>[2x]MFKFIGCGSAFNTRLGNNSAYIKEDGILFMIDCGSANFDRIMRSDLLEGVEDIVVLMTHTHPDHVGSLGDLIFYSYFCMGQVKVPNLTVYAPYDMKIS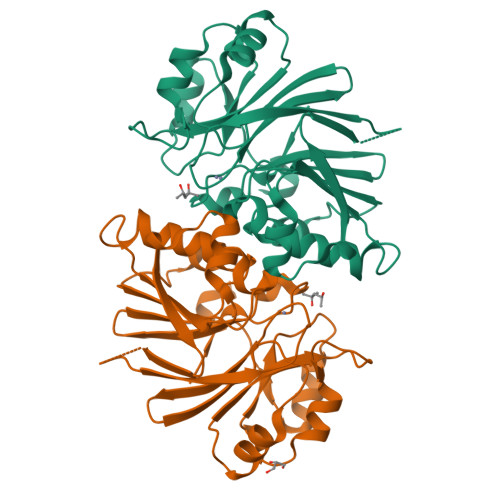KVLQGMGVERECYRLIQFDNSNEYPPGFHKDGFHIKFQVVPNRHVPELLCYGYLITYKDKTIYYSGDANNISPFILRMLEDGEIDYFYQDTCQADYEGNVHLSLKKLSEMVWANRDRVYCMHLDGGFNREQAEELGFNVVQPSYKFMI> MTTLTRQDLNSAQVV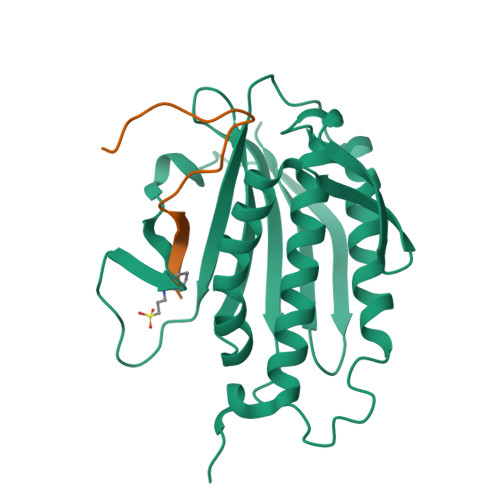ADVLSEFLEVAVHLILYVREVYPVGIFQKRKKYNVPVQMSCHPELNQYIQDTLHCVKPLLEKNDVEKVVVVILDKEHRPVEKFVFEITQPPLLSINSDSLLSHVEQLLRAFILKISKVDKVLDHNPPGCTFTVLVHTREAATRNMEKIQVIKDFPWILADEQDVHMHDPRLIPLKTMTSDILKMQLYVEERAHKNS;> MSASSGPWKPAKPAPSVSPGPWKPIPSVS ECF transporters consist of two identical or highly similar cytoplasmic ATPases, EcfA and EcfA′, and two transmembrane subunits, EcfT and the S-component124. The membrane-embedded S-component serves as both the substrate-binding and the substrate-translocation domain. The other three subunits (EcfA, EcfA′ and EcfT) together form the ECF module that energizes substrate transport by the S-component456. Here we report crystal structures of the group II ECF transporter for folate from Lactobacillus delbrueckii (L. delbrueckii) in the apo-state and in complex with the slowly hydrolysable ATP analogue AMP–PNP.

We determined crystal structures of the ECF–FolT2 complex from L. delbrueckii in the apo state (no nucleotides or folate) and in an AMP–PNP-bound state at 3.0 and 3.3 Å resolution, respectively. Two patches of well-defined electron density were observed in EcfA and EcfA′ of the complex crystallized in the presence of Mg–AMP–PNP and were assigned to the nucleotide molecules. The two AMP–PNP molecules interact with conserved motifs that are essential for ATP binding and hydrolysis in other ABC transporters. The AMP–PNP molecules interact only with motifs from a single ATPase subunit, and are separated from the signature motifs (LSGGQ) on the other subunit. Therefore the ATP hydrolysis sites are still incomplete. Even though AMP–PNP molecules are bound to both subunits, binding does not lead to the closed conformation of the ATPases. In the AMP–PNP structure it is packed tightly against the FolT subunit and interacts with the loops L3 and the C terminus of H5, but in the apo structure it has hinged away and the two membrane proteins interact less tightly. The position of the L1 loop in the complexes is stabilized by a hydrogen bond between the backbone carbonyl group of G35 and the highly conserved R196 (the AMP–PNP structure) or N189 (in the apo structure) in the coupling domain of EcfT. The loss of the high-affinity binding site for folate in the complex explains why no electron density for folate was found in the structure of the AMP–PNP-bound complex even though a high concentration of the substrate was added during crystallization. Our structural work shows that the binding of AMP–PNP to ECF–FolT2 is not sufficient to form the closed EcfA–EcfA′ dimer.

>[2x]MHHHHHHHHHHGENLYFQGSDNIISFDHVTFTYPDSPRPALSDLSFAIERGSWTALIGHNGSGKSTVSKLINGLLAPDDLDKSSITVDGVKLGADTVWEVREKVGIVFQNPDNQFVGATVSDDVAFGLENRAVPRPEMLKIVAQAVADVGMADYADSEPSNLSGGQKQRVAIAGILAVKPQVIILDESTSMLDPEGKEQILDLVRKIKEDNNLTVISITHDLEEAAGADQVLVLDDGQLLDQGKPEEIFPKVEMLKRIGLDIPFVYRLKQLLKERGIVLPDEIDDDEKLVQSLWQLNS;>[2x]MAIKFENVSYVYSPGSPLEAIGLDQLNFSLEEGKFIALVGHTGSGKSTLMQHFNALLKPTSGKIEIAGYTITPETGNKGLKDLRRKVSLAFQFSEAQLFENTVLKDVEYGPRNFGFSEDEAREAALKWLKKVGLKDDLIEHSPFDLSGGQMRRVALAGVLAYEPEIICLDEPAAGLDPMGRLEMMQLFKDYQAAGHTVILVTHNMDDVADYADDVLALEHGRLIKHASPKEVFKDSEWLQKHHLAEPRSARFAAKLEAAGLKLPGQPLTMPELADAIKQSLKGGEHE;>MKSESKVSSKLELRELVLLAMVIAIKVILGQFKVGNATLQVGLGFIGSVMLGYLFGPWWGFAGGALSDLVSSVIFGNLGGFFIGFTLTAALGPMIYGFFLYKQPIQIWRVIASVICVTVICNIGLNTLWVSMMYGINFMVALSSRILKEMITPWIQMVAVWFILEGLSRVKLSRKFWSHPQFEK[2x];>[2x]MSKIIIGRYLPGTTFVYRVDPRAKLLTTFYFIIMIFLANNWVSYLVISIFGLAYVFATGLKARVFWDGVKPMIWMIVFTSLLQTFFMAGGKVYWHWWIFTLSSEGLINGLYVFIRFAMIILVSTVMTVTTKPLEIADAMEWMLTPLKLFKVNVGMISLVISIALRFVPTLFDQTVKIMNAQRSRGADFNDGGLVKRAKSVVPMLVPLFIDSLEVALDLSTAMESRGYKGSEGRTRYRILEWSKVDLIPVAYCLLLTILMITTRKH> ETSYTLNEVVPLKEFVPEWVRIGFSATTGAEFAAHEVLSWYF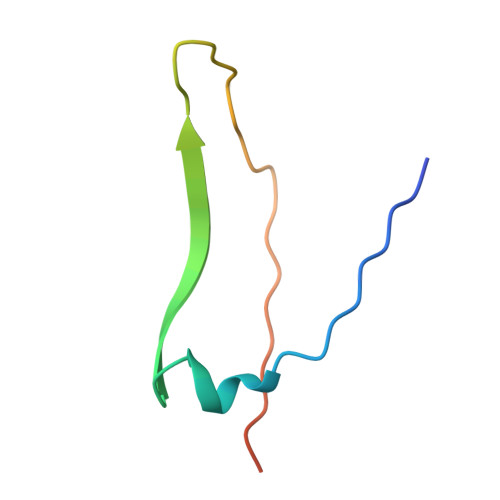HSELAGTSSS>PIELLPETPSQTAGPYVHIGLALEAAGNPTRDQEIWNRLAKPDAPGEHILLLGQVYDGNGHLVRDSFLEVWQADANGEYQDAYNLENAFNSFGRTATTFDAGEWTLHTVKPGVVNNAAGVPMAPHINISLFARGINIHLHTRLYFDDEAQANAKCPVLNLIEQPQRRETLIAKRCEVDGKTAYRFDIRIQGEGETVFFDF[3x];>[3x]PAQDNSRFVIRDRNWHPKALTPDYKTSIARSPRQALVSIPQSISETTGPNFSHLGFGAHDHDLLLNFNNGGLPIGERIIVAGRVVDQYGKPVPNTLVEMWQANAGGRYRHKNDRYLAPLDPNFGGVGRCLTDSDGYYSFRTIKPGPHPWRNGPNDWRPAHIHFGISGPSIATKLITQLYFEGDPLIPMCPIVKSIANPEAVQQLIAKLDMNNANPMDCLAYRFDIVL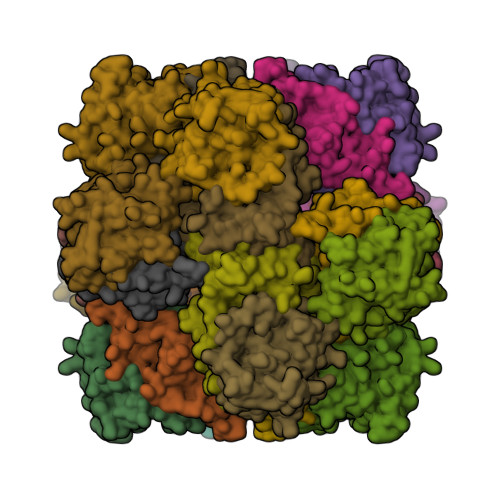RGQRKTHFENC>[6x]GAMGSIQENLIFPMDNPKGIDGFTNLKEKDIATNENKLLRTITADKMIPAFLITPISSQIAGKVIAQVESDIFAHMGKAVLI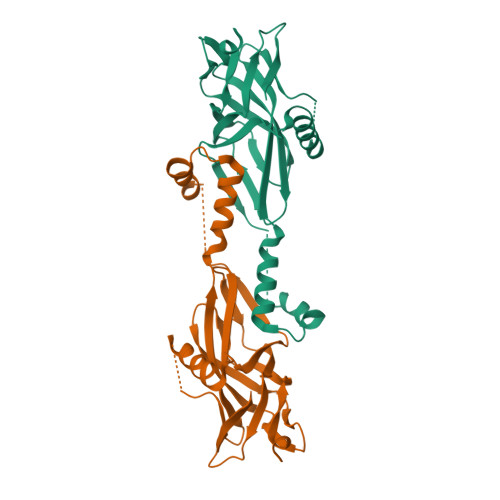PKGSKVIGYYSNNNKMGEYRLDIVWSRIITPHGINIMLTNAKGADIKGYNGLVGELIERNFQRYGVPLLLSTLTNGLLIGITSALNNRGNKEGATNFFGDYLLMQLMRQSGMGINQVVNQILRDKSKIAPIVVIREGSRVFISPNTDIFFPIPRENEVIAEFLK Avapritinib is the only potent and selective inhibitor approved for the treatment of D842V-mutant gastrointestinal stromal tumors (GIST), the most common primary mutation of the platelet-derived growth factor receptor α (PDGFRA). Against this background, we solve the crystal structures of avapritinib in complex with wild-type and mutant PDGFRA and stem cell factor receptor (KIT), which provide evidence and understanding of inhibitor binding and lead to the identification of a sub-pocket (Gα-pocket). Furthermore, we report the identification of a sub-pocket (Gα-pocket) located in the N-lobe of the kinase domain, which is surrounded by amino acids of key regulatory elements such as the Gly-rich loop and the αC-helix.

Previously, we found that mutation of the gatekeeper PDGFRA-Thr674 to a non-polar isoleucine (T674I) or a sterically more demanding arginine (T674R) induces resistance to avapritinib. The complex crystal structure of avapritinib bound to PDGFRA-T674I demonstrated, as anticipated by Grunewald et al., that avapritinib binds an active-like kinase conformation, which is characterized by an extended AL and a DFG-in state as was evident from Asp836 (or Asp810 in KIT) of the Asp-Phe-Gly (DFG) motif pointing into the ATP-binding site. Avapritinib interacts with the hinge region via H-bonding with the backbone amine of Cys677 via the pyrrolotriazine scaffold N2 nitrogen. The scaffold further interacts with Leu599, Leu825, Ala625, and Tyr676. The solvent-exposed methyl pyrazole undergoes a cation-π-interaction with Arg597. The linking piperazine forms contacts with Val607 and Cys835, while the pyrimidine interacts with Val607 and forms an additional hydrogen bond with the catalytic Lys627. For the primary amine located at the stereocenter, we observed an ionic interaction between the primary amine and Asp836 from the DFG motif. The binding of avapritinib stabilizes the DFG-in conformation of the kinase domain in which the amino acids Gly605 and Val607 of the Gly-rich loop, Leu641 of the αC-helix, the catalytic Lys627 and Leu629 form a hydrophobic pocket that can perfectly accommodate the shape of the fluorobenzene moiety of the inhibitor. Additional cation-π interactions of the fluorobenzene were observed with the catalytic Lys627. This pocket extends beyond the phosphate-binding region of the ATP-binding site and is distinct from the backpocket (often referred to as the switch or deep pocket in some publications) and has not been targeted or studied previously in the field of KIT and PDGFRA or related kinases; therefore, we refer to this structural feature as the Gα-pocket, to account for its location between the αC-helix and Gly-rich loop.

> KQKPRYEIRWRVIESISPDGHEYIYVDPMQLPYDSRWEFPRDGLVLGRVLGSGAFGKVVEGTAYGLSRSQPVMKVAVKMLKPTARSSEKQALMSELKIMTHLGPHLNIVNLLGACTKSGPIYIIIEYCFYGDLVNYLHKNRDSFLSHKKKSMLDSEVKNLLSDDNSEGLTLLDLLSFTYQVARGMEFLASKNCVHRDLAARNVLLAQGKIVKICDFGLARDIMHDSNYVSKGSTFLPVKWMAPESIFDNLYTTLSDVWSYGILLWEIFSLGGTPYPGMMVDSTFYNKIKSGYRMAKPDHATSEVYEIMVKCWNSEPEKRPSFYHLSEIVENLLPGQYKKSYEKIHLDFLKSD> VFPSDATFGMGDRVRKKSGAAWQGQIVGWYCTNLTPEGYAVESEAHPGSVQI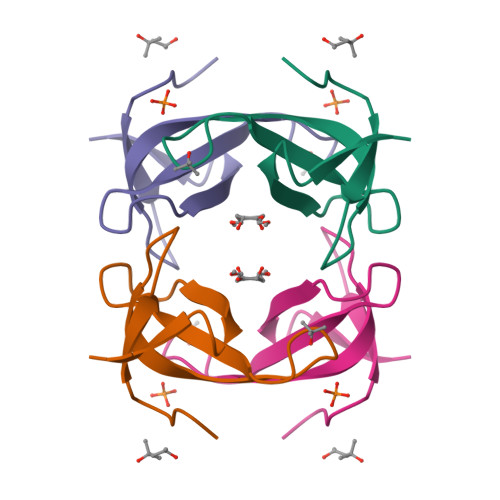YPVAALERIN(4~{R})-~{N}-[3-(7-methoxy-3,4-dihydro-2~{H}-quinolin-1-yl)propyl]-4-methyl-2-oxidanylidene-1,3,4,5-tetrahydro-1,5-benzodiazepine-6-carboxamide 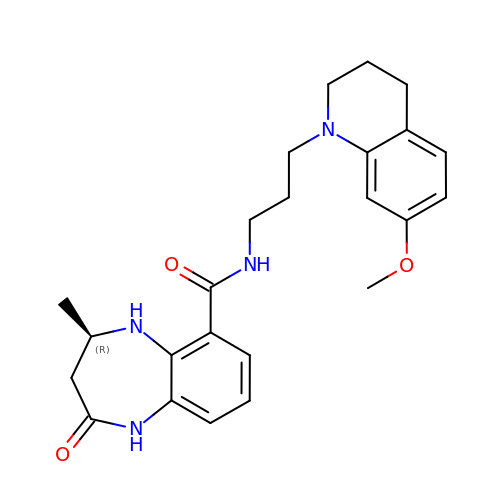| C24 H30 N4 O3 | XZQSPHYHBYGJPB-MRXNPFEDSA-N3-{5-[(2E,4aR,7aR)-6-benzoyl-2-imino-3-methyl-4-oxooctahydro-7aH-pyrrolo[3,4-d]pyrimidin-7a-yl]thiophen-3-yl}benzonitrile 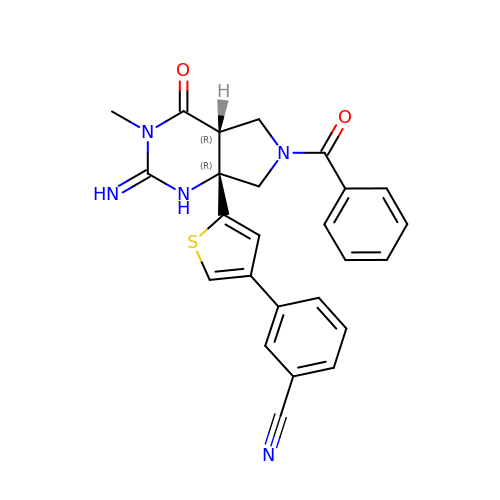| C25 H21 N5 O2 S | POOXGNGZUXTIQE-CPJSRVTESA-N4-((4,5-dihydro-1H-imidazol-2-yl)amino)-N-(4-((4,5-dihydro-1H-imidazol-2-yl)amino)phenyl)benzamide dihydrochloride 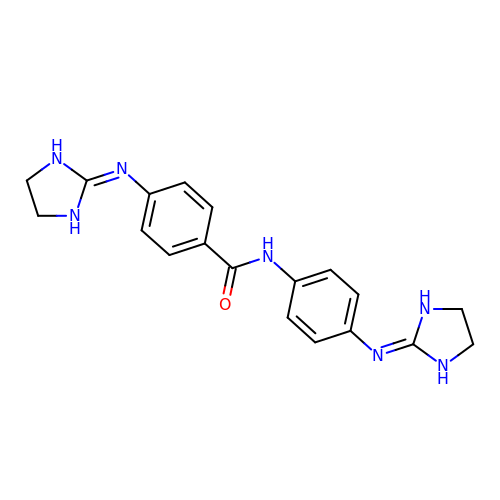| C19 H21 N7 O | LDJIXMMIBFEFIF-UHFFFAOYSA-N>SDAQEILSRLNSVLEAAWKTILNLASATDAAEKAYKEGREEDLATYLDQAASYQSQVDQYAVETVRLLAELKKVFPDEEADRALQIAEKLLKTVQEASKTLDTAVAAAANGDEETFAKAFNQFVSLGNQAD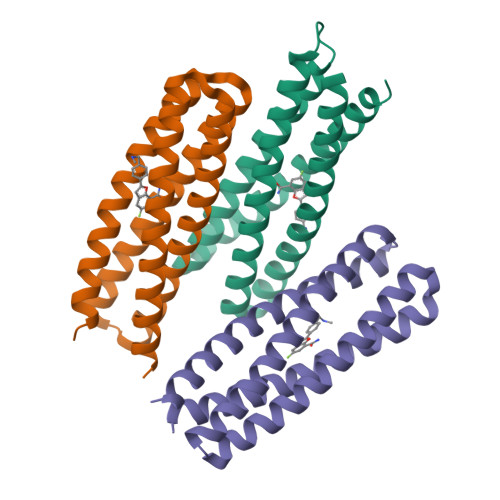TLFTQLQRTLTNLNKK[3x]> MNSQTDYTNYIIFNPEGKIKQLEFINNTVQLGSTVVALKNKSFGVFVTYNEKRSKFALQQKKIFPINSKSLFSFSGITNDGTKIVKYLKNSTVFENIRKGRDIHPIHVFDDLCYSACIRTLTNGNRLYGVQGLLLTDYQGISLVLFDPKGSAKEVRG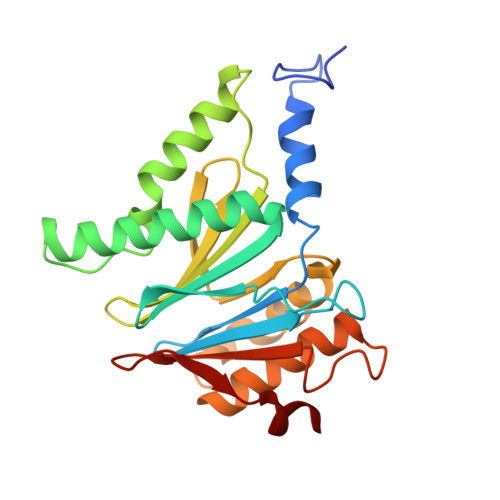MSIGSRSQSCRTILEDECDKFEEYNKEELVRLGIKALRNAYPETGVLNKDNVDIWILETNQESKQIKSEEYLQ> IPTCKITLKETFLTSPEELYRVFTTQELVQAFTHAPATLEADRGGKFHMVDGNVSGEFTDLVPEKHIVMKWRFKSWPEGHFATITLTFIDKNGETELCMEGRGIPAPEEERTRQGWQRYYF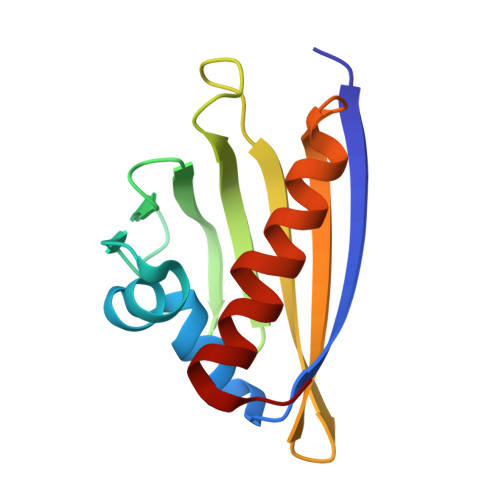EGIKQTFGYGA> IESIIKTATDTVKSEINAELGVVPSLNAVETGATSNTEPEEAIQTRTVINQHGVSETLVENFLSRAALVSKRSFEYKDHTSSAAQTDKNFFKWTINTRSFVQLRRKLELFTYLRFDAEITILTTVAVNGSSNNTYVGLPDLTLQAMFVPTGALTPEKQDSFHWQSGSNASVFFKISDPPARMTIPFMCINSAYSVFYDGFAGFEKSGLYGINPADTIGNLCVRIVNEHQPVGFTVTVRVYMKPKHIKAWAPRPPRTLPYMSIANANYKGKGRAPNALNAIIGNRDSVKTMPHNIVTT;> RVLQLKLGNSAIVTQEAANYCCAYGEWPNYLPDHEAVAIDKPTQPETATDRFYTLRSVKWEAGSTGWWWKLPDALNNIGMFGQNVQHHYLYRSGFLIHVQCNATKFHQGALLVVAIPEHQRGAHNTNTSPGFDDIMKGEEGGTFNHPYVLDDGTSLACATIFPHQWINLRTNNSATIVLPWMNAAPMDFPLRHNQWTLAIIPVVPLGTRTMSSMVPITVSIAPMCCEFNGLRHAITQ;> GVPTYLLPGSGQFLTTDDHSSAPVLPCFNPTPEMHIPGQVRNMLEVVQVESMMEINNTESAVGMERLKVDISALTDVDQLLFNIPLDIQLDGPLRNTLVGNISRYYTHWSGSLEMTFMFCGSFMATGKLILCYTPPGGSCPTTRETAMLGTHVVWDFGLQSSVTLIIPWISGSHYRMFNNDAKSTNANVGYVTCFMQTNLIVPSESSDTCSLIGFIAAKDDFSLRLMRDSPDIGQLDHL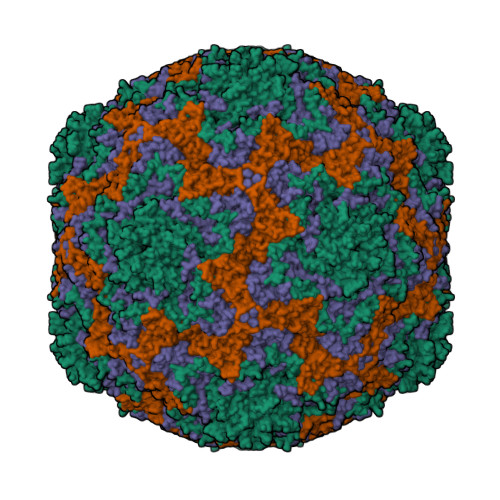HAAEAAYQ;> QINFYKDSYAASASKQDFSQDPSKFTEPVV>MATLFQVSMGSMRHRRNGNFESSRLLYSSMSR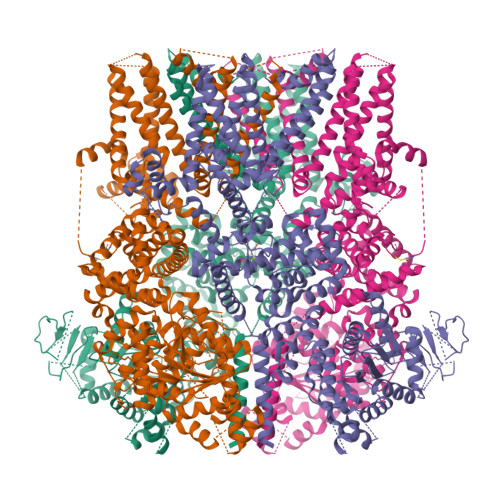SIDVACSDADLANFIQENFKKRECVFFTKDTKSMGNLCKCGYPENQHIEGTQVNTTEKWNYKKHXXXXXXXXXXXXXXXXXXXXXKYIRLSCDTDSETLYDLMTQHWHLKTPNLVISVTGGAKNFALKPRMRKIFSRLIYIAQSKGAWIFTGGTHYGLMKYIGEVVRDNTISRSSEENVVAIGIAAWGMISNRETLIRTADSDGSYLAHYIMDDLKRDPLYCLDNNHTHLLLVDNGTHGHPTIEAKVRTQLEKYISERVIPESNYGGKIPIVCFAQGGGKETLKSINVAIKSKIPCVVVEGSGRIADVIASLVEAEGTLASSCVKESLLRFLPRTISRLSEEETESWIKWIKEVLESPHLLTVIKIEEAGDEIVSNAISFALYKAFSTNEHDRDNWNGQLKLLLEWNQLDLASDEIFTNDRNWESADLQDVMFTALVKDRPKFVRLFLENGLNLRKFLTTEVLRELYTNNFSSLVFKNLQIAKNSYNDALLTFVWKMVEDFRRGAKRDDKNSKDEMEIELSEECPITRHPLQALFIWSVLQNKKELSKVIWEQTRGCTLAALGASKLLKSMAKVKNDINAAGESEELANEYETRAVELFTECYSNDEDLAEQLLTYSCEAWGGSNCLELAVEARDQQFIAQPGVQNFLSKQWYGEISRDTKNWKIILCLFFFPLIGCGFISFRKKPVEKTKKLFLYYVSFFTSPFVVFSWNVIFYIAFLLLFAYVLLMDFQKEPTALEIILYVLVFILLCDEVRQWYMNGSKYFSDLWNVMDTLGIFYFIAGIVFRLHSDESSWYSGRVIFCLDYIVFTLRLIHIFTVSRNLGPKIIMLQRMMIDVFFFLFLFAVWMVAFGVARQGILRKNEHRWEWIFRSVIYEPYLAMFGQYPDDIDGTTYNFDHCTFSGNESKPLCVELDANNQPRFPEWITIPLVCIYMLSTNILLVNLLVAMFGYTVGSVQENNDQVWKFQRFFLVQEYCSRLTIPFPFVIFAYIFMVMRKCFKCCCKKESKEPSVCCSRNEDNEILAWEAVMKENYLVKINTKASDSSEEXXXXXXXXXXXXXXXXXXXXXXXXSNSLEVLFQGPDYKDDDDKAHHHHHHHHHH[4x]>[2x]MLPHGLIVSCQALPDEPLHSSFIMSKMALAAYEGGAVGIRANTKEDILAIKETVDLPVIGIVKRDYDHSDVFITATSKEVDELIESQCEVIALDATLQQRPKETLDELVSYIRTHAPNVEIMADIATVEEAKNAARLGFDYIGTTLHGYTSYTQGQLLYQNDFQFLKDVLQSVDAKVIAEGNVITPDMYKRVMDLGVHCSVVGGAITRPKEITKRFVQIMED

The third step in the sialic acid catabolic pathway is mediated by the enzyme N-acetylmannosamine-6-phosphate 2-epimerase (NanE), which catalyzes an inversion of stereochemistry at the C2 position of N-acetylmannosamine-6-phosphate (ManNAc-6P), yielding N-acetylglucosamine-6-phosphate (GlcNAc-6P). The crystal structure of NanE from Staphylococcus aureus, which comprises a triosephosphate isomerase barrel fold with an unusual dimeric architecture, was solved with both natural and modified substrates. NanE is essential for the growth of S. aureus in media containing N-acetylneuraminic acid as the sole carbon source and has a highly conserved active site across both Gram-positive and Gram-negative bacteria. Based on our structural and kinetic data, we propose that NanE performs its epimerization reaction using a novel proton displacement mechanism mediated by the substrate.

We determined the crystal structure of SaNanE to evaluate the reaction mechanism in the S. aureus homolog. Purified recombinant protein (see Experimental procedures section) readily produced crystals that diffracted to a maximum resolution of 1.84 Å. SaNanE crystallized with two monomers in the asymmetric unit. The monomeric structure of SaNanE is illustrated in Figure 2A (β-strands labeled i–viii and α-helices labeled A–H), showing that it assembles into a classic triosephosphate isomerase (TIM) barrel fold, with one exception: α-helix H does not pack against the β-barrel but instead mediates dimerization between the monomers. Unlike other TIM-barrel enzymes, dimerization between the SaNanE monomers is enabled by a C-terminal α-helix, which projects away from each barrel and packs against the neighboring monomer. The theoretical scattering profile calculated for the wildtype crystal structure of SaNanE was a good fit for the experimental scattering data (χ2 = 0.56), suggesting that the crystal structure is an accurate representation of the solution structure. In general, the active-site residues map to regions of the protein that have low temperature factors, as evidenced by an overlay of active-site residues on the temperature factor plot for each chain in the asymmetric unit. To further gauge the dynamics of the active-site residues, we conducted an ensemble refinement of the structure and again found that the active-site residues have low root-mean-square fluctuations and largely occupy a single conformation. In the apo structure, two active-site residues have side-chain moieties with significantly perturbed pKa values: Lys63 has a predicted pKa of 8.0, considerably lower than the pKa for lysine in water (10.4), whereas Glu180 has a predicted pKa of 7.1, which is considerably higher than the pKa for glutamic acid in water (4.5). The carboxylate group of Glu180 points toward the plane of the guanidinium group (3.2 Å) of the conserved Arg40, which may explain the perturbed pKa.> KNNINKTRMNDLNREETRLKTFTDWPLDWLDKRQLAQTGMYFTHAGDKVKCFFCGVEIGSWEQEDQPVPEHQRWSPNCPLLRRRTTNNVPINAEALDRILPPI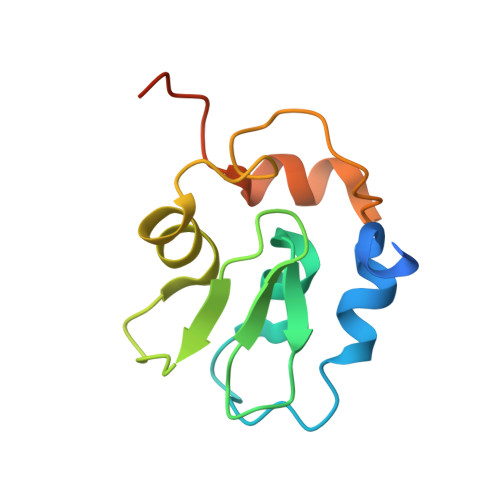SYDICGANDSTLE> MPQTAGPDTIRILVSTDNHVGYEERDPIRKDDSWRTFDEIMQLARTKDVDMVLLGGDLFHDNKPSRKAMYQVMRSLRKNCLGMKPCELEFLSDPAEVFEGAFPHVNYYDPDINVSIPVFSIHGNHDDPSGDGHLCSLDLLQVAGLVNYFGRVPEADNIHVKPILLQKGKTKLALYGMSNVRDERIHRTFRDNKVRFYRPSQQTGDWFNLLTLHQNHYAHTPTGYLSENMLPDFLDLVIWGHEHECLIDPKKNPETGFHVMQPGSSIATSLVPGEAVPKHIAILSITGKSFEVEKIPLRTVRPFVIREITLATDKRFKGLEKKQDNRQEVTKRLMQIVEEMIAEANEMWRSLHEDSQDDEDEEQPLPLIRLKVEYSSPEGTKFEVENPQRFSNRF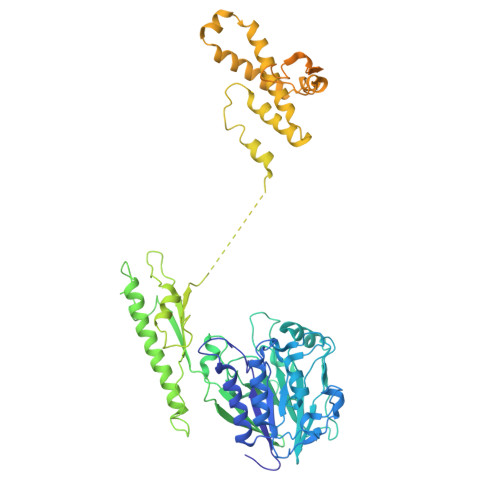AGKVANQNDVVHFYRKKTGTTRKPKEGKRELPEGIAEALEDSDSISVDALVQEFFAQQSLKILPQAPFGDAVNQFVSKDDKHAVEMFVMDSLSSQVRGLLQLDDDKINEGLDSHIEDFRKVMEKNFLSGQQKQAQRRRRFKEKPEGWDSDLNGHWTLQPEAIEELSSSPEPAKEGGRVRPASRITVGDEDNLFEEEEFVQKTTAKRAPTTRATRKTAAATRATTATKASAPAKKSIAAPRGRKRANPFQDSAEEEEDVIMDDDDDYKPAPPVKAPPPKPARETQTRGAPKTRQTTLNFSQAERPTRTTQKAIEISDDEISEDDAFESMPARKSKRY>MSQPITRENFDEWMIPVYAPAPFIPVRGEGSRLWDQQGKEYIDFAGGIAVNALGHAHPELREALNEQASKFWHTGNGYTNEPVLRLAKKLIDATFADRVFFCNSGAEANEAALKLARKFAHDRYGSHKSGIVAFKNAFHGRTLFTVSAGGQPAYSQDFAPLPADIRHAAYNDINSASALIDDSTCAVIVEPIQGEGGVVPASNAFLQGLRELCNRHNALLIFDEVQTGVGRTGELYAYMHYGVTPDLLTTAKALGGGFPVGALLATEECARVMTVGTHGTTYGGNPLASAVAGKVLELINTPEMLNGVKQRHDWFVERLNTINHRYGLFSEVRGLGLLIGCVLNADYAGQAKQISQEAAKAGVMVLIAGGNVVRFAPALNVSEEEVTTGLDRFAAACEHFVSRGSS[4x]

Escherichia coli possesses two acyl ornithine aminotransferases, one catabolic (AstC) and the other anabolic (ArgD), that participate in L-arginine metabolism. The arginine-succinyl transferase pathway of E. coli provides nitrogen for growth via a series of succinylated intermediates. In conclusion, the E. coli AstC protein, involved in arginine catabolism, is a PLP containing transaminase that is structurally similar to the related protein ArgD, which is the transaminase enzyme used in arginine synthesis. From the biochemical data, it appears that AstC and ArgD are biochemically similar, consistent with the ability of astC to complement an argD deletion. Both have comparable steady state kinetic values, with a strong preference for the acylated ornithine derivatives AO (AstC and ArgD) and SO (for AstC, at least) over ORN itself.

To better understand the intricacies of the reaction, ORN, αKG and GLU were soaked into crystals of holo-AstC. We were also unable to find extra electron density for the ORN soaked crystals, but there was a distinct change in the active site, with the PLP-Schiff base bond to Lys252 clearly broken. This finding is consistent with the completion of the first half reaction (i.e. deamination of the substrate), producing an aldehyde and pyridoxamine. The electron density is set at 1.5 sigma. Figure 5B shows the density for PLP and Lys252 after the crystals were soaked with ORN. The lack of internal aldimine in the ArgD structures is similar to the structure of AstC after soaking with ORN, suggesting that the majority of St-ArgD had undergone a half reaction. SO, ORN and AO were docked into the active site of the structure with PLP covalently bound to Lys252, while αKG was docked into the non-covalently bound pyridoxamine phosphate structure. We see that αKG is positioned with the ketone carbon ready for attack by the amino nitrogen of pyridoxamine phosphate. Additionally, the carbonyl group is stabilized by interactions with Arg141.> ESLYQSKYEELQITAGRHGDSVRNSKIEISELNRVIQRLRS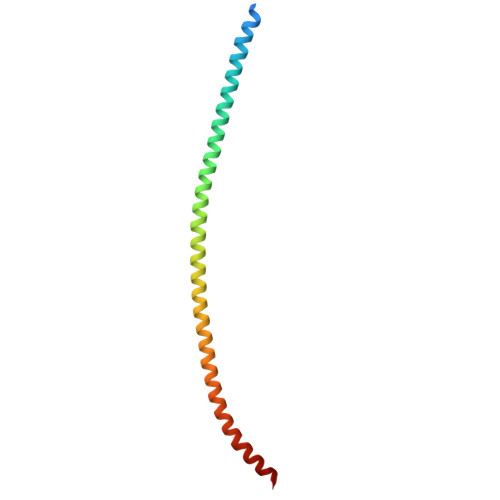EIDNVKKQISNLQQSISDAEQRGENALKDAKNKLNDLEDALQQAKEDLARLLRDYQELMNTKLALDLEIATYRTLLEGE>ANEVIKCKAAVAWEAGKPLSIEEIEVAPPKAHEVRIKIIATAVCHTDAYTLSGADPEGCFPVILGHEGAGIVESVGEGVTKLKAGDTVIPLYIPQCGECKFCLNPKTNLCQKIRVTQGKGLMPDGTSRFTCKGKTILHYMGTSTFSEYTVVADISVAKIDPLAPLDKVCLLGCGISTGYGAAVNTAKLEPGSVCAVFGLGGVGLAVIMGCKVAGASRIIGVDINKDKFARAKEFGATECINPQDFSKPIQEVLIEMTDGGVDYSFECIGNVKVMRAALEACHKGWGVSVVVGVAASGEEIATRPFQLVTGRT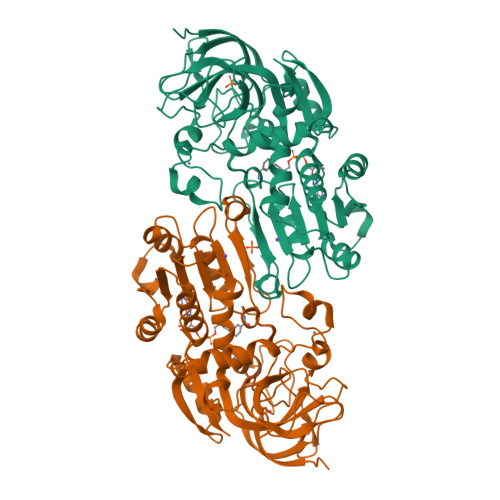WKGTAFGGWKSVESVPKLVSEYMSKKIKVDEFVTHNLSFDEINKAFELMHSGKSIRTVVKI[2x]> ADPESCTFKISLRNFRSILSWELKNHSIVPTHYTLLYTIMS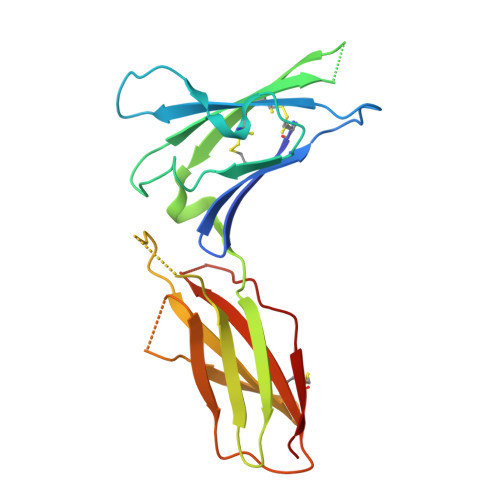KPEDLKVVKNCANTTRSFCDLTDEWRSTHEAYVTVLEGFSGNTTLFSCSHNFWLAIDMSFEPPEFEIVGFTNHINVMVKFPSIVEEELQFDLSLVIEEQSEGIVKKHKPEIKGNMSGNFTYIIDKLIPNTNYCVSVYLEHSDEQAVIKSPLKCTLLPP> ISEFDYKDHEIDYKDDDDKWIMSLSIKELYYTKDKSINNVNLADGNYVVNRGDGWILS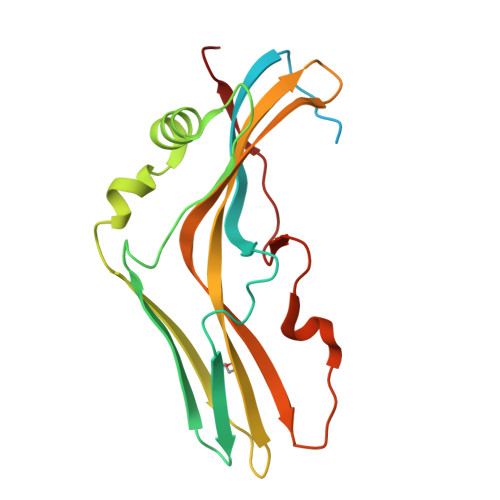RQNQNLGGNISNNGCTAIVGDLRIRETATPYYYPTASFNEEYIKNNVQNVFANFTEASEIPIGFEFSKTAPSNKSLYMYLQYTYIRYEIIKVLQNTVTERAVLYVPSLGYVKSIEFNSEEQIDKNFYFTSQDKCILNEKFIYKKIDD>[2x]SNAEDTFKVGLIVPMTGGQASTGKQIDNAIKLYIKKHGDTVAGKKIEVILKDDAAIPDNTKRLAQELIVNDKVNVIAGFGITPAALAAAPLATQAKVPEIVMAAGTSIITERSPYIVRT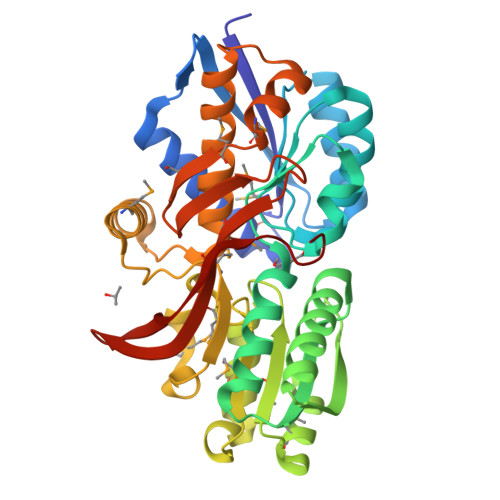SFTLAQSSIIIGDWAAKNGIKKVATLTSDYAPGNDALAFFKERFTAGGGEIVEEIKVPLANPDFAPFLQRMKDAKPDAMFVFVPAGQGGNFMKQFAERGLDKSGIKVIGPGDVMDDDLLNSMGDAALGVVTAHMYSAAHPSAMNKEFVAAYKKEFGQRPGFMAVGGYDGIHLVFEALKKTGGKADGDSLIAAMKGMKWESPRGPISIDPETRDIVQNIYIRKVEKVDGELYNIEFAKFDAVKDPGKTKK> MGSSHHHHHHSSGENLYFQHMPFAARLNTPMGPGRTVVVKGEVNANAKSFNVDLLAGKSKDIALHLNPRLNIKAFVRNSFLQE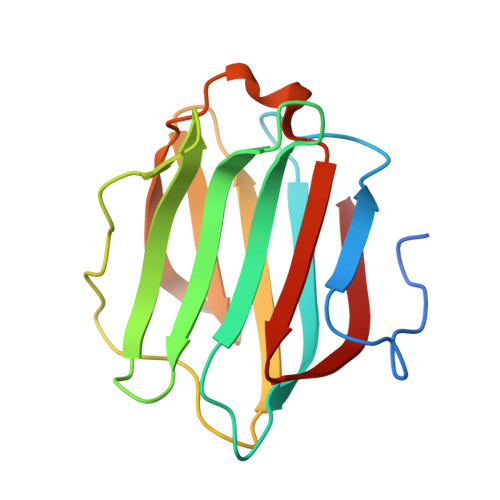SWGEEERNITSFPFSPGMYFEMIIYCDVREFKVAVNGVHSLEYKHRFKELSSIDTLEINGDIHLLEVRSW2-[(2R,3S,4R,5R)-1-[3-(4-fluorophenyl)propyl]-5-(hydroxymethyl)-3,4-bis(oxidanyl)pyrrolidin-2-yl]-N-methyl-ethanamide 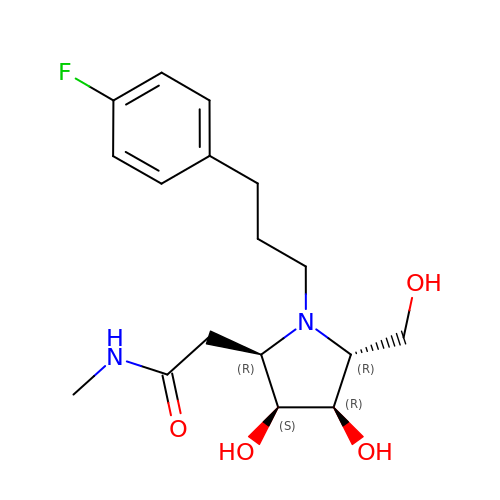| C17 H25 F N2 O4 | IVSNKOONVYNOFH-TXCZRRACSA-N> GPHMTDPITNYKP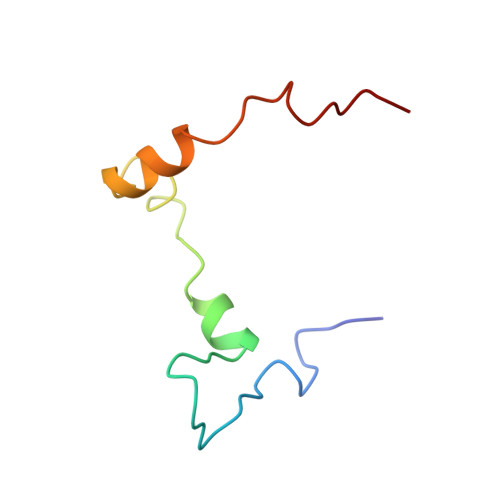MDLQYKTYAYSMNELYHLKPSLASASYEEDPLISELVRSLPKRKFWRLRMG>GSEELLDLFNRQVTQEFTASQVYLSASIWFDQNDWEGMAAYMLAESAEEREHGLGFVDFANKRNIPIELQAVPAPVSCAEWSSPEDVWQSILELEQANTRSLLNLAEAASTCHDFAVMAFLNPFHLQQVNEEDKIGSILAKVTDENRTPGLLRSLDVVSFLG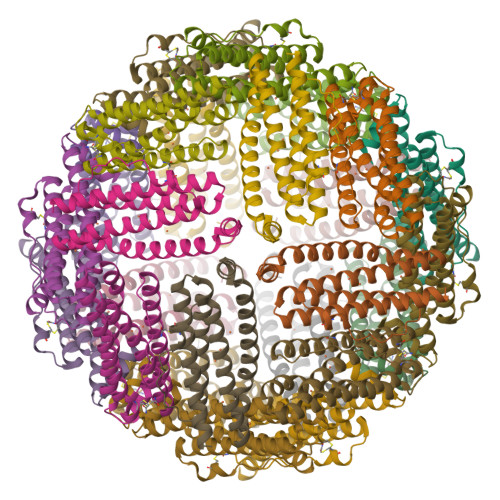PCLFRS[6x]>MKKILIIGGVAGGASAAARARRLSETAEIIMFERGEYVSFANCGLPYHISGEIAQRSALVLQTPESFKARFNVEVRVKHEVVAIDRAAKLVTVRRLLDGSEYQESYDTLLLSPGAAPIVPPIPGVDNPLTHSLRNIPDMDRILQTIQMNNVEHATVVGGGFIGLEMMESLHHLGIKTTLLELADQVMTPVDREMAGFAHQAIRDQGVDLRLGTALSEVSYQVQTHVASDAAGEDTAHQHIKGHLSLTLSNGELLETDLLIMAIGVRPETQLARDAGLAIGELGGIKVNAMMQTSDPAIYAVGDAVEEQDFVTGQACLVPLAGPANRQGRMAADNMFGREERYQGTQGTAICKVFDLAVGATGKNEKQLKQAGIAFEKVYVHTASHASYYPGAEVVSFKLLFDPVKGTIFGAQAVGKDGIDKRIDVMAVAQRAGMTVEQLQHLELSYAPPYGSAKDVINQAAFVASNIIKGDATPIHFDQIDNLSEDQLLLDVRNPGELQNGGLEGAVNIPVDELRDRMHELPKDKEIIIFCQVGLRGNVAYRQLVNNGYRARNL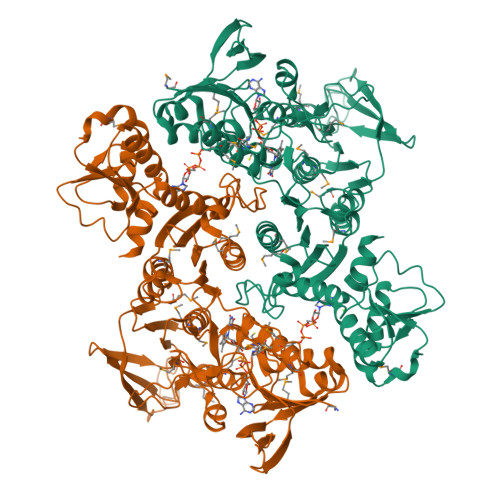IGGYRTYKFASVLEHHHHHH[2x]>[2x]RECSLTGEWTNDLGSNMTIGAVNSDGEFTGTYITAVTATSNEIKESPLHGTENTINKR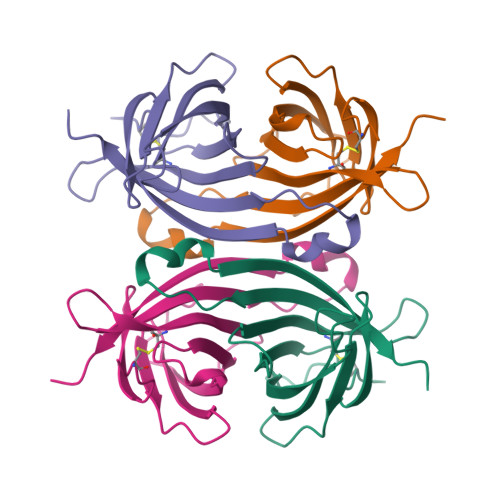TQPTFGFTVNWKFSESTTVFTGQCFIDRNGKEVLKTMWLLRSSVNDIGDDWKATRVGINIFTRLLTQKE> MGYYDIDDVLADGTEFPCKFQYDIPGLGYLENNPGRPITKNTKLSLPLWLARILAIVGGDEALVDEEPVPFVELLPPDMFSTKVMNAIKTDPVALDLHSINSHFFSLAIKWIMLFS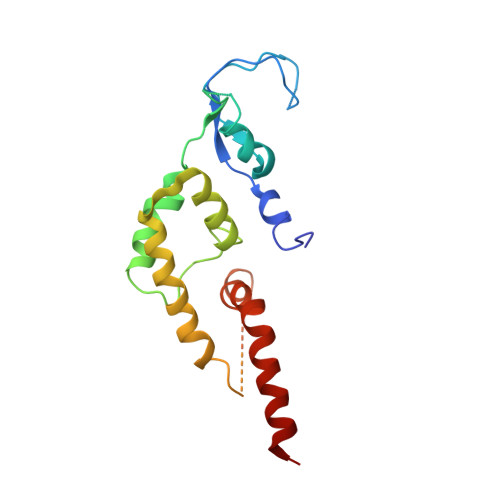EKELANVVSELLLQRAQELNHHASSLSIDLNADSTGKNSANTNIATSTFLLKLEEMEKEIYKKSHESYKDTKRWMFKK>GHMEAIKGSDV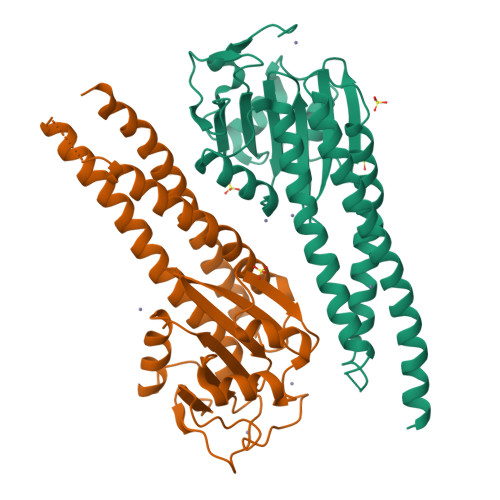NVPDAVFAWLLDGRGGVKPLEDNDVIDSQHPCWLHLNYTHPDSARWLASTPLLPNNVRDALAGESSRPRVSRMGEGTLITLRCINGSTDERPDQLVAMRLYMDERFIVSTRQRKVLALDDVVSDLQEGTGPVDCGGWLVDVCDALTDHASEFIEELHDKIIDLEDNLLDQQIPPRGFLALLRKQLIVMRRYMAPQRDVYARLASERLPWMSDDHRRRMQDIADRLGRGLDEIDACIARTGIMADEIAQVMQES[2x]> MIIVYTTF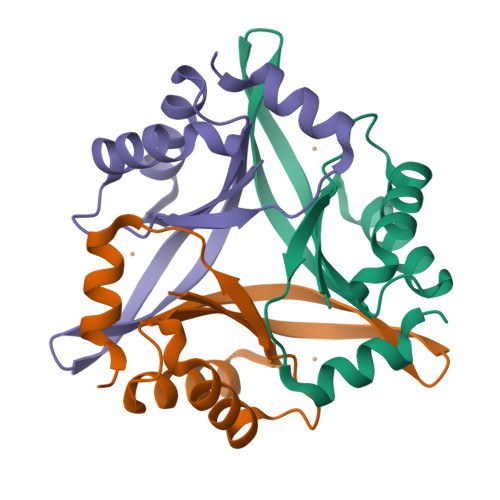PDWESAEKVVKTLLKERLIACANLREHRAFYWWEGKIEEDKEVGAILKTREDLWEELKERIKELHPYDVPAIIRIDVDDVNEDYLKWLIEETKK>MKIEEVKSTTKTQRIASHSHVKGLGLDESGLAKQAASGLVGQENAREACGVIVELIKSKKMAGRAVLLAGPPGTGKTALALAIAQELGSKVPFCPMVGSEVYSTEIKKTEVLMENFRRAIGLRIKETKEVYEGEVTELTPCETENPMGGYGKTISHVIIGLKTAKGTKQLKLDPSIFESLQKERVEAGDVIYIEANSGAVKRQGRCDTYATEFDLEAEEYVPLPKGDVHKKKEIIQDVTLHDLDVANARPQGGQDILSMMGQLMKPKKTEITDKLRGEINKVVNKYIDQGIAELVPGVLFVDEVHMLDIECFTYLHRALESSIAPIVIFASNRGNCVIRGTEDITSPHGIPLDLLDRVMIIRTMLYTPQEMKQIIKIRAQTEGINISEEALNHLGEIGTKTTLRYSVQLLTPANLLAKINGKDSIEKEHVEEISELFYDAKSSAKILADQQDKYMK[3x];>[3x]MATVTATTKVPEIRDVTRIERIGAHSHIRGLGLDDALEPRQASQGMVGQLAARRAAGVVLEMIREGKIAGRAVLIAGQPGTGKTAIAMGMAQALGPDTPFTAIAGSEIFSLEMSKTEALTQAFRRS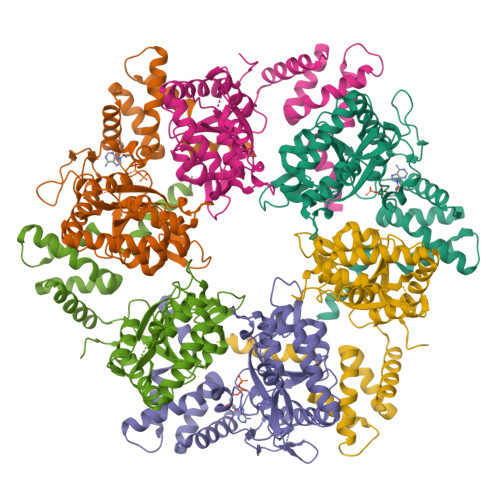IGVRIKEETEIIEGEVVEIQIDRPATGTGSKVGKLTLKTTEMETIYDLGTKMIESLTKDKVQAGDVITIDKATGKISKLGRSFTRARDYDAMGSQTKFVQCPDGELQKRKEVVHTVSLHEIDVINSRTQGFLALFSGDTGEIKSEVREQINAKVAEWREEGKAEIIPGVLFIDEVHMLDIESFSFLNRALESDMAPVLIMATNRGITRIRGTSYQSPHGIPIDLLDRLLIVSTTPYSEKDTKQILRIRCEEEDVEMSEDAYTVLTRIGLETSLRYAIQLITAASLVCRKRKGTEVQVDDIKRVYSLFLDESRSTQYMKEYQDAFLFNELKGETMDTS> VDIAAFDPDKDGTIDLKEALAAGSAAFDKLDPDKDGTLDAKELKGRVSEADLKKLDPDNDGTLDKK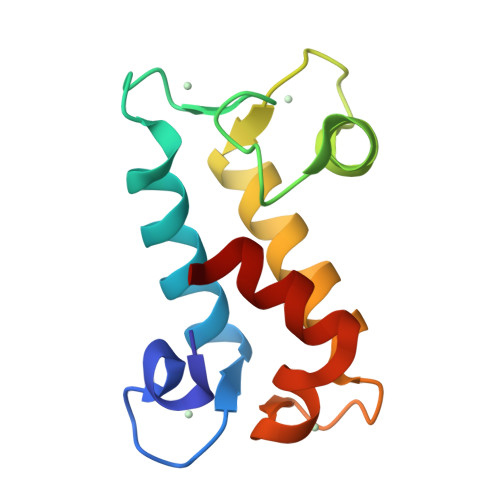EYLAAVEAQFKAANPDNDGTIDARELASPAGSALVNLIR> MKILHTSDWHLGVTSWTSSRPVDRREELKKALDKVVEEAEKREVDLILLTGDLLHSRNNPSVVALHDLLDYLKRMMRT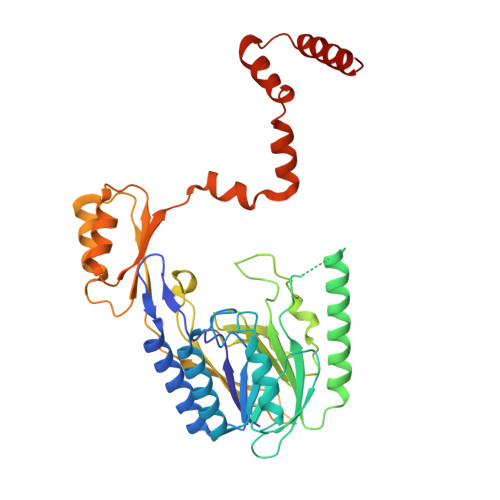APVVVLPGNQDWKGLKLFGNFVTSISSDITFVMSFEPVDVEAKRGQKVRILPFPYPDESEALRKNEGDFRFFLESRLNKLYEEALKKEDFAIFMGHFTVEGLAGYAGIEQGREIIINRALIPSVVDYAALGHIHSFREIQKQPLTIYPGSLIRIDFGEEADEKGAVFVELKRGEPPRYERIDASPLPLKTLYYKKIDTSALKSIRDSCRNFPGYVRVVYEEDSGILPDLMGEIDNLVKIERKSRREIEEVLRESPEEFKEELDKLDYFELFKEYLKKREENHEKLLKILDELLDEVKKSEA> MSTVPELLARQVTRAPDAVAVVDRDRVLTYRELDELAGRLSGRLIGRGVRRGDRVAVLLDRSADLVVTLLAIWKAGAAYVPVDAGYPAPRVAFMVADSGASRMVCSAATRDGVPEGIEAIVVTDEEAFEASAAGARPG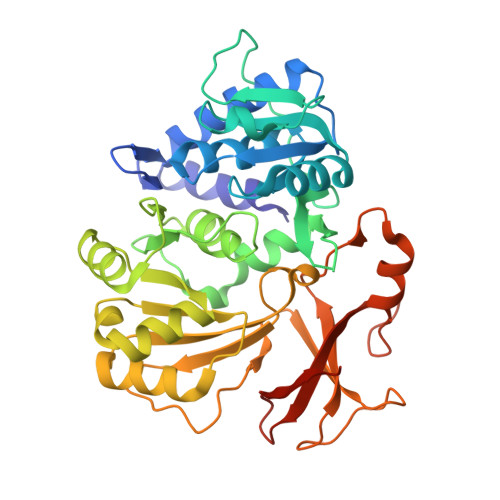DLAYVMYTSGSTGIPKGVAVPHRSVAELAGNPGWAVEPGDAVLMHAPYAFDASLFEIWVPLVSGGRVVIAEPGPVDARRLREAISSGVTRAYLTAGSFRAVAEESPESFAGLREVLTGGDVVPAHAVARVRSACPRVRIRHLYGPTETTVCATWHLLEPGDEIGPVLPIGRPLPGRRAQVLDASLRAVAPGVIGDLYLSGAGLADGYLRRAGLTAERFVADPSAPGARMYRTGDLAQWTADGALLFAGRADDQGSHHHHHH[2-({2-[bis(2-phosphonoethyl)amino]ethyl}[2-(6-oxo-3,6-dihydro-9H-purin-9-yl)ethyl]amino)ethyl]phosphonic 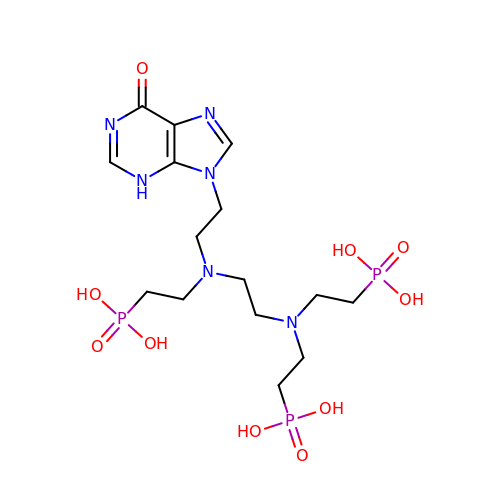acid | C15 H29 N6 O10 P3 | JHLUHXHQASLZGD-UHFFFAOYSA-N> MGSDYKDHDGDYKDHDIDYKDDDDKGSGSLEVLFQGPMDPIINGNSANVYLTDSYLKGVISFSECNALGSYIFNGPYLKNDYTNLISRQNPLIEHMNLKKLNITQSLISKYHKGEIKLEEPTYFQSLLMTYKSMTSSEQIATTNLLKKIIRRAIEISDVKVYAILNKLGLKEKDKIKSNNGQDEDNSVITTIIKDDILSAVKDNQSHLKADKNHSTKQKDTIKTTLLKKLMCSMQHPPSWLIHWFNLYTKLNNILTQYRSNEVKNHGFTLIDNQTLSGFQFILNQYGCIVYHKELKRITVTTYNQFLTWKDISLSRLNVCLITWISNCLNTLNKSLGLRCGFNNVILTQLFLYGDCILKLFHNEGFYIIKEVEGFIMSLILNITEEDQFRKRFYNSMLNNITDAANKAQKNLLSRVCHTLLDKTVSDNIINGRWIILLSKFLKLIKLAGDNNLNNLSELYFLFRIFGHPMVDERQAMDAVKINCNETKFYLLSSLSMLRGAFIYRIIKGFVNNYNRWPTLRNAIVLPLRWLTYYKLNTYPSLLELTERDLIVLSGLRFYREFRLPKKVDLEMIINDKAISPPKNLIWTSFPRNYMPSHIQNYIEHEKLKFSESDKSRRVLEYYLRDNKFNECDLYNCVVNQSYLNNPNHVVSLTGKERELSVGRMFAMQPGMFRQVQILAEKMIAENILQFFPESLTRYGDLELQKILELKAGISNKSNRYNDNYNNYISKCSIITDLSKFNQAFRYETSCICSDVLDELHGVQSLFSWLHLTIPHVTIICTYRHAPPYIGDHIVDLNNVDEQSGLYRYHMGGIEGWCQKLWTIEAISLLDLISLKGKFSITALINGDNQSIDISKPIRLMEGQTHAQADYLLALNSLKLLYKEYAGIGHKLKGTETYISRDMQFMSKTIQHNGVYYPASIKKVLRVGPWINTILDDFKVSLESIGSLTQELEYRGESLLCSLIFRNVWLYNQ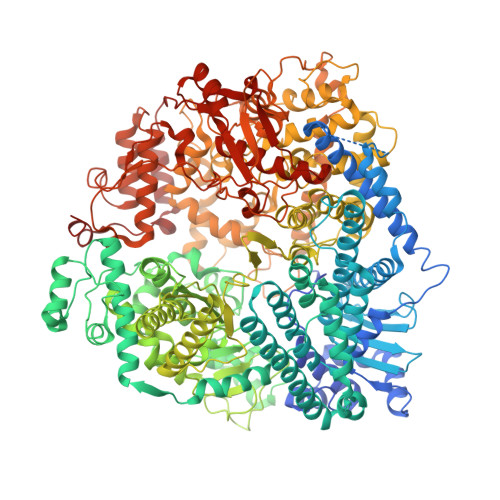IALQLKNHALCNNKLYLDILKVLKHLKTFFNLDNIDTALTLYMNLPMLFGGGDPNLLYRSFYRRTPDFLTEAIVHSVFILSYYTNHDLKDKLQDLSDDRLNKFLTCIITFDKNPNAEFVTLMRDPQALGSERQAKITSEINRLAVTEVLSTAPNKIFSKSAQHYTTTEIDLNDIMQNIEPTYPHGLRVVYESLPFYKAEKIVNLISGTKSITNILEKTSAIDLTDIDRATEMMRKNITLLIRILPLDCNRDKREILSMENLSITELSKYVRERSWSLSNIVGVTSPSIMYTMDIKYTTSTISSGIIIEKYNVNSLTRGERGPTKPWVGSSTQEKKTMPVYNRQVLTKKQRDQIDLLAKLDWVYASIDNKDEFMEELSIGTLGLTYEKAKKLFPQYLSVNYLHRLTVSSRPCEFPASIPAYRTTNYHFDTSPINRILTEKYGDEDIDIVFQNCISFGLSLMSVVEQFTNVCPNRIILIPKLNEIHLMKPPIFTGDVDIHKLKQVIQKQHMFLPDKISLTQYVELF>KVLFVCIHNTARSVMAEALFNAMAKSWKAESAGVEKAERVDETVKRLLAERGLKAKEKPRTVDEVNLDDFDLIVTVCEESSCVVLPTDKPVTRWHIEN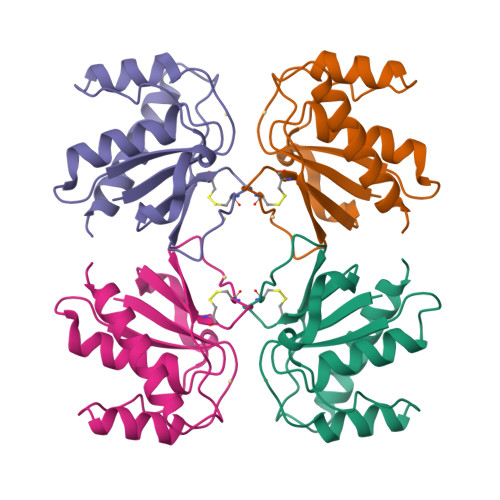PAGKDEGTYRRVLAEIEERVKKLVGE[4x]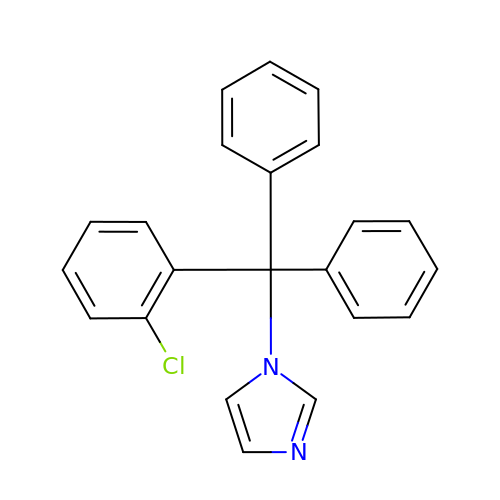1-[(2-CHLOROPHENYL)(DIPHENYL)METHYL]-1H-IMIDAZOLE | C22 H17 Cl N2 | VNFPBHJOKIVQEB-UHFFFAOYSA-N> SSVFVPDEWEVSR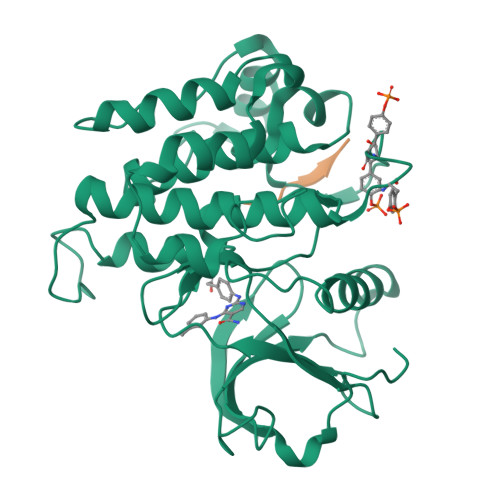EKITLLRELGQGSFGMVYEGNARDIIKGEAETRVAVKTVNESASLRERIEFLNEASVMKGFTCHHVVRLLGVVSKGQPTLVVMELMAHGDLKSYLRSLRPEAENNPGRPPPTLQEMIQMAAEIADGMAYLNAKKFVHRDLAARNCMVAHDFTVKIGDFGMTRDIYETDYYRKGGKGLLPVRWMAPESLKDGVFTTSSDMWSFGVVLWEITSLAEQPYQGLSNEQVLKFVMDGGYLDQPDNCPERVTDLMRMCWQFNPKMRPTFLEIVNLLKDDLHPSFPEVSFFHSEENK;> DYMNMS>SPNYDKWEMERTDITMKHKLGGGQYGEVYEGVWKKYSLTVAVKTLKEDTMEVEEFLKEAAVMKEIKHPNLVQLLGVCTREPPFYIITEFMTYGNLLDYLRECNRQEVNAVVLLYMATQISSAMEYLEKKNFIHRDLAARNCLVGENHLVKVADFGLSRLMTGDTYTAHAGAKFPIKWTAPESLAYNKFSIKSDVWAFGVLLWEIATYGMSPYPGIDLSQVYELLEKDYRMERPEGCPEKVYEL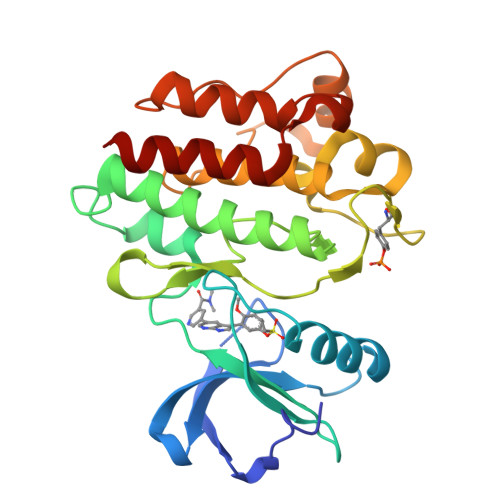MRACWQWNPSDRPSFAEIHQAFETMFQES[2x]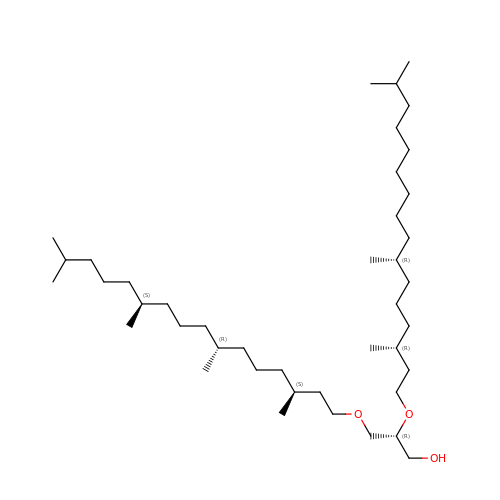1-[2,6,10.14-TETRAMETHYL-HEXADECAN-16-YL]-2-[2,10,14-TRIMETHYLHEXADECAN-16-YL]GLYCEROL | C42 H86 O3 | YERVUJAKCNBGCR-BIHSMRAKSA-N(1~{S})-1-[(3,4-dimethoxyphenyl)methyl]-6,7-dimethoxy-1,2,3,4-tetrahydroisoquinoline 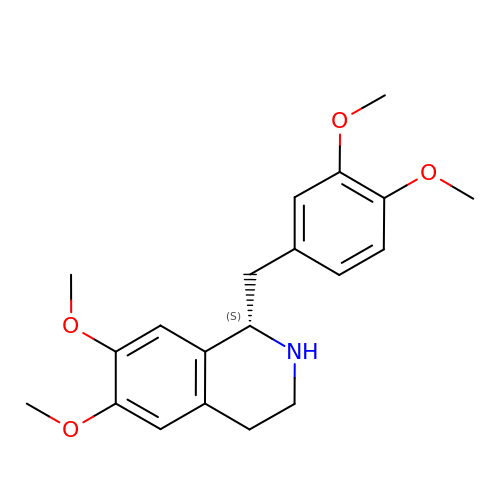| C20 H25 N O4 | YXWQTVWJNHKSCC-INIZCTEOSA-N> MTDAAEEVLLGKKGCTGVITLNRPKFLNALTLNMIRQIYPQLKKWEQDPETFLIIIKGAGGKAFCAGGDIRVISEAEKAKQKIAPVFFREEYMLNNAVGSCQKPYVALIHGITMGGGVGLSVHGQFRVATEKCLFAMPETAIGLFPDVGGGYFLPRLQGKLGYFLALTGFRLKGRDVYRAGIATHFVDSEKLAMLEEDLLALKSPSKENIASVLENYHTES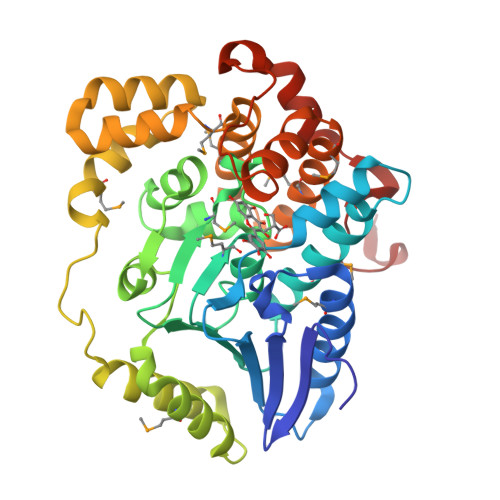KIDRDKSFILEEHMDKINSCFSANTVEEIIENLQQDGSSFALEQLKVINKMSPTSLKITLRQLMEGSSKTLQEVLTMEYRLSQACMRGHDFHEGVRAVLIDKDQSPKWKPADLKEVTEEDLNNHFKSLGSSDLKFAENLYFQ>GCGTAUA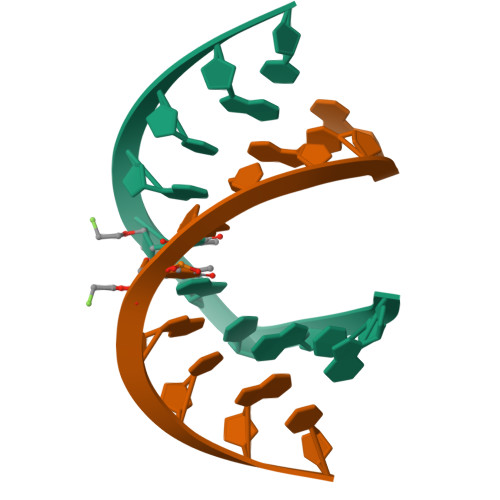CGC[2x]> SKTIVLSVGEATRTLTEIQSTADRQIFEEKVGPLVGRLRLTASLRQNGAKTAYRV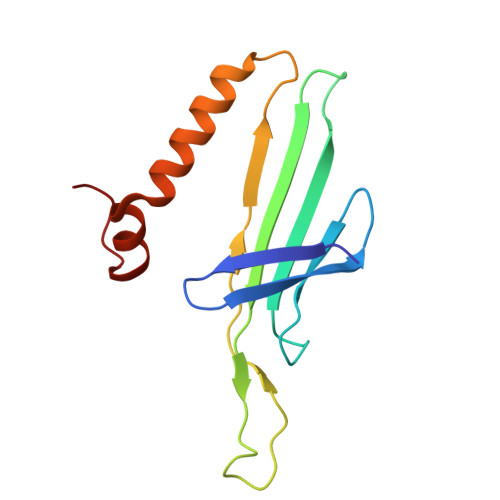NLKLDQADVVDCSTSVCGELPKVRYTQVWSHDVTIVANSTEASRKSLYDLTKSLVATSQVEDLVVNLVPLGR> MAIASEFSSLPSYAAFATAQEAYEQAVANGDSEVVLKKLKKSLNVAKSEFDRDAAMQRKLEKMADQAMTQMYKQARSEDKRAKVTSAMQTMLFTMLRKLDNDALNNIINNARDGCVPLNIIPLTTAAKLMVVIPDYNTYKNT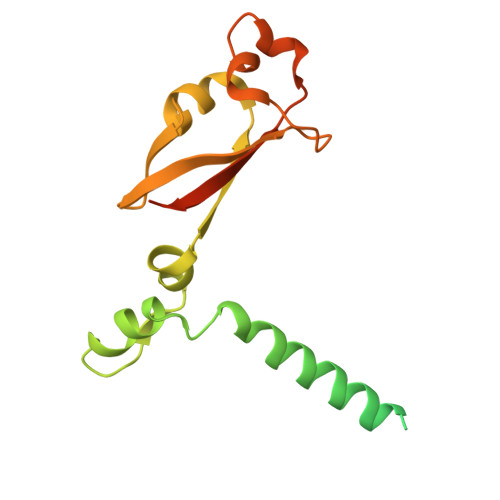CDGTTFTYASALWEIQQVVDADSKIVQLSEISMDNSPNLAWPLIVTALRANSAVKLQHHHHHHHH>MDNSHDSDSVFLYHIPCDNCGSSDGNSLFSDGHTFCYVCEKWTAGNEDTKERASKRKPSGGKPMTYNVWNFGESNGRYSALTARGISKETCQKAGYWIAKVDGVMYQVADYRDQNGNIVSQKVRDKDKNFKTTGSHKSDALFGKHLWNGGKKIVVTEGEIDMLTVMELQDCKYPVVSLGHGASAAKKTCAANYEYFDQFEQIILMFDMDEAGRKAVEEAAQVLPAGKVRVAVLPCKDANECHLNGHDREIMEQVWNAGPWIPDGVVSALSLRERIREHLSSEESVGLLFSGCTGINDKTLGARGGEVIMVTSGSGMGKSTFVRQQALQWGTAMGKKVGLAMLQESVEETAEDLIGLHNRVRLRQSDSLKREIIENGKFDQWFDELFGNDTFHLYDSFAEAETDRLLAKLAYMRSGLGCDVIILDHISIVVSASGESDERKMIDNLMTKLKGFAKST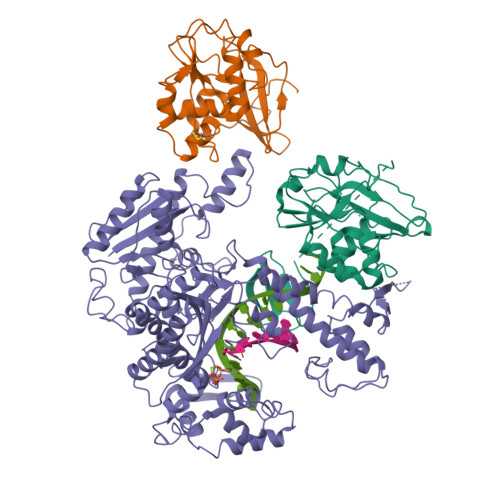GVVLVVICHLKNPDKGKAHEEGRPVSITDLRGSGALRQLSDTIIALERNQQGDMPNLVLVRILKCRFTGDTGIAGYMEYNKETGWLEPSSYSGEEESHSESTDWSNDTDF[2x];> MIVSDIEANALLESVTKFHCGVIYDYSTAEYVSYRPSDFGAYLDALEAEVARGGLIVFHNGHKYDVPALTKLAKLQLNREFHLPRENCIDTLVLSRLIHSNLKDTDMGLLRSGKLPGKRFGSHALEAWGYRLGEMKGEYKDDFKRMLEEQGEEYVDGMEWWNFNEEMMDYNVQDVVVTKALLEKLLSDKHYFPPEIDFTDVGYTTFWSESLEAVDIEHRAAWLLAKQERNGFPFDTKAIEELYVELAARRSELLRKLTETFGSWYQPKGGTEMFCHPRTGKPLPKYPRIKTPKVGGIFKKPKNKAQREGREPCELDTREYVAGAPYTPVEHVVFNPSSRDHIQKKLQEAGWVPTKYTDKGAPVVDDEVLEGVRVDDPEKQAAIDLIKEYLMIQKRIGQSAEGDKAWLRYVAEDGKIHGSVNPNGAVTGRATHAFPNLAQIPGVRSPYGEQCRAAFGAEHHLDGITGKPWVQAGIDASGLELRCLAHFMARFDNGEYAHEILNGDIHTKNQIAAELPTRDNAKTFIYGFLYGAGDEKIGQIVGAGKERGKELKKKFLENTPAIAALRESIQQTLVESSQWVAGEQQVKWKRRWIKGLDGRKVHVRSPHAALNTLLQSAGALICKLWIIKTEEMLVEKGLKHGWDGDFAYMAWVHDEIQVGCRTEEIAQVVIETAQEAMRWVGDHWNFRCLLDTEGKMGPNWAICH>[2x]GKQLTILGST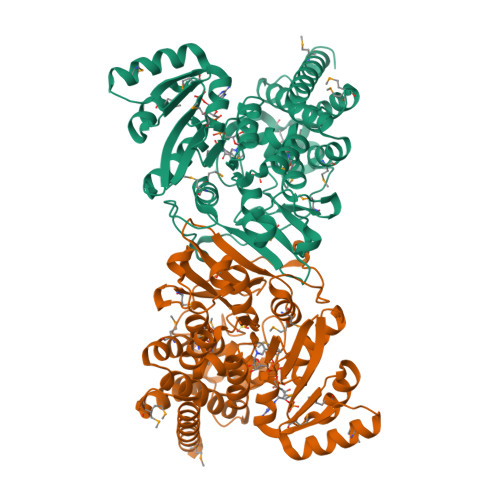GSIGCSTLDVVRHNPEHFRVVALVAGKNVTRMVEQCLEFSPRYAVMDDEASAKLLKTMLQQQGSRTEVLSGQQAACDMAALEDVDQVMAAIVGAAGLLPTLAAIRAGKTILLANKESLVTCGRLFMDAVKQSKAQLLPVDSEHNAIFQSLPQPIQHNLGYADLEQNGVVSILLTGSGGPFRETPLRDLATMTPDQACRHPNWSMGRKISVDSATMMNKGLEYIEARWLFNASASQMEVLIHPQSVIHSMVRYQDGSVLAQLGEPDMRTPIAHTMAWPNRVNSGVKPLDFCKLSALTFAAPDYDRYPCLKLAMEAFEQGQAATTALNAANEITVAAFLAQQIRFTDIAALNLSVLEKMDMREPQCVDDVLSVDANAREVARKEVMRLASSA> MDMHMIVKVVAILAVLFLVYKLWESMNKPNASPLKIQNPYEKYMNSAEGGEYDAEDDDIY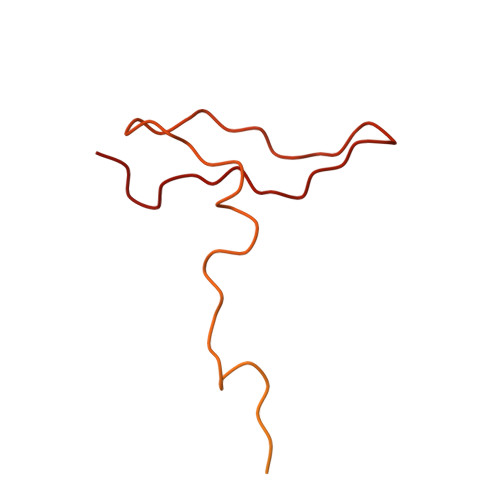YPETDAEDDDIYTGETDDMYDGEDDDIYVQEGDDIEDAEDEPYDDSADMEQDVPKVQQPMMPLLTPSSQLLPKPSPEAADFAQFAPKNLQAQNFLTATQWIGVNTQGSSLKNANYDLRADPIIPKADVGPWMMSSVDPNIYQKPLFG Here, isolation of the dominant isoform of haemoglobin from Atlantic cod caught in southwest Norway is reported and its X-ray crystal structure is presented. The full genome of Atlantic cod has been sequenced, and about 70 isoforms of haemoglobin have been proposed by the EST translation of the genome. However, sequence similarity within the α and β forms of cod haemoglobin is high, simplifying the structure-identification research challenge. The potential use of haemoglobin adducts as potential biomarkers of PAH exposure in Atlantic cod is under investigation in our research group.

The best data were collected to 2.5 Å resolution from a crystal of approximately 0.3 × 0.05 × 0.05 mm in size on beamline ID23-1 at the ESRF. The crystal belonged to space group P212121, with unit-cell parameters a = 62, b = 103, c = 199 Å. A homology model of tetrameric cod haemoglobin (made for pre-crystallographic studies) was used as a template for structure determination using molecular replacement. Phaser was able to identify two tetramers in the asymmetric unit [Fig. 3(a)]. The two cod haemoglobin tetramers superimpose on each other with an r.m.s.d. of 0.51 Å. Differences in conformation are primarily located in the loop between residues 45–60 and the C-terminal loops. Eight heme groups could be located in the electron density. The heme iron appears to be pentacoordinated in all subunits. The side chains of the histidines in the α and β units have conformations similar to that observed for perch haemoglobin, with distances of about 4.0–4.4 and 2.1–2.3 Å between the histidinyl N∊2 atom and Fe for α-chain residues His60 and His89, respectively, and 4 and 2.1–2.4 Å for β-chain residues His64 and His93, respectively. Haemoglobins from cold-adapted species have been found to follow distinct autooxidation patterns. The small differences in the distances and the amount of difference density observed close to the heme iron may suggest different states of autooxidation. The cod haemoglobin structure presented in this work appears to have Ala at position 63 and Leu at position 56 in the β chains, instead of Lys or Met, which are more common in cod sequences.

>[4x]XSLSSKQKATVKDFFSKMSTRSDDIGAEALSRLVAVYPQTKSYFSHWKDASPGSAPVRKHGITIMGGVYDAVGKIDDLKGGLLSLSELHAFMLRVDPVNFKLLAHCMLVCMSMIFPEEFTPQVHVAVDKFLAQLALALAEKYR;>VEWTDSERAIITSIFSNLDYEEIGRKSLCRCLIVYPWTQRYFGAFGNLYNAETILANPLIAAHGTKILHGLDRALKNMDDIKNTYAELSLLHSDKLHVDPDNFRLLADCLTVVIAAKMGSAFTVDTQVAWQKFLSVVVSALGRQY[4x]>[5x]GAMADREKLLTESGVYGTFATFQMDHDWWDLPGESRVISVAEVKGLVEQWSGKILVESYLLRGLSD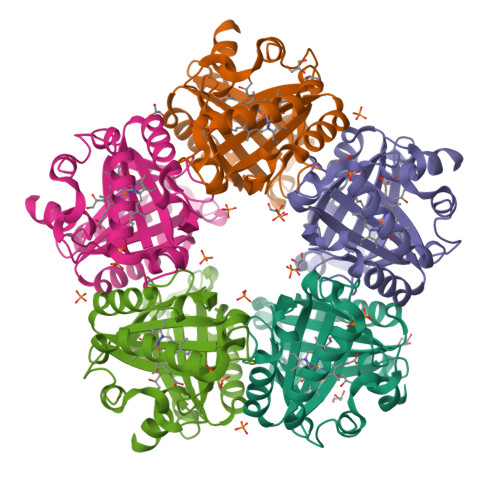HADLMFRVHARTLSDTQQFLSAFMGTRLGRHLTSGGLLHGVSKKPTYVAGFPESMKTELQVNGESGSRPYAIVIPIKKDAEWWALDQEARTALMQEHTQAALPYLKTVKRKLYHSTGLDDVDFITYFETERLEDFHNLVRALQQVKEFRHNRRFGHPTLLGTMSPLDEILEKFAQ>RSPWARWFPKTLPCDVTLDVSKNHVIVDCTDKHLTEIPGGIPTNTTNLTLTINHIPDISPASFHRLVHLVEIDFRCNCVPIRLGSKSNMCPRRLQIKPRSFSGLTYLKSLYLDGNQLLEIPQGLPPSLQLLSLEANNIFSIRKEQLTELANIEILYLGQNCYYRNPCYVSYSIEKDAFLNLTKLKVLSLKDNNVTTVPTVLPSTLTELYLYNNMIAEIQEDDFNNLNQLQILDLSGNCPRCYNAPFPCTPCKNNSPLQIPVNAFDALTELKVLRLHSNSLQHVPPRWFKNINNLQELDLSQNFLAKEIGDAKFLHFLPNLIQLDLSFNFELQVYRASMNLSQAFSSLKSLKILRIRGYVFKELKSFQLSPLHNLQNLEVLDLGTNFIKIANLSMFKQFKRLKVIDLSVNKISPSGDSLVPRGSSNARTSVESYEPQVLEQLYYFRYDKYARSCRFKNKEASFTSVQESCYKYGQTLDLSKNSIFFIKSSDFQHLSFLKCLNLSGNLISQTLNGSEFQPLAELRYLDFSNNRLDLLHSTAFEELRKLEVLDISSNSHYFQSEGITHMLNFTKNLKVLQKLMMNDNDISSSTSRTMESESLRTLEFRGNHLDVLWRDGDNRYLQLFKNLLKLEELDISKNSLSFLPSGVFDGMPPNLKNLSLAKNGLKSFIWEKLRYLKNLETLDLSHNQLTTVPERLSNCSRSLKNLILKNNQIRSLTKYFLQDAFQLRYLDLSSNKIQMIQKTSFPENVLNNLKMLLLHHNRFLCTCDAVWFVWWVQHTEVTIPYLATDVTCVGPGAHKGQSVISLDLYTCELDLTNEFLVPR[2x]

TLR7 recognizes pathogenic single-stranded RNAs (ssRNAs) and plays a crucial role in the innate immune response to viral infections, such as human immunodeficiency virus 1 and influenza virus. The activated TLR7 dimer contains two distinct ligand-binding sites. Small-molecule agonists, including imiquimod, guanosine and 2’,3’-cGMP bind to site 1 in the dimerization interface and directly induce the formation of the activated TLR7 dimer, while uridine-containing ssRNAs bind to site 2 and allosterically enhance the binding affinity of site 1 ligands for TLR73,4. Using cryo-electron microscopy (cryo-EM) combined with X-ray crystallography, we reveal that the structural equilibrium between open and closed conformations that underlies TLR7 antagonism.

We have previously reported a series of 8-oxoadenine derivatives (8-OAs) represented by Cpd-1, Cpd-2, and Cpd-3 as specific TLR7 agonists. We confirmed the binding mode of 8-OAs by crystallography. The potent agonist Cpd-3 induced almost complete dimerization under both neutral and acidic conditions. The TLR7/Cpd-3 complex exclusively adopted a closed-form conformation which is in good agreement with the crystal structure. Three agonists Cpd-1, Cpd-2, and Cpd-3 had higher binding energy in the closed form than the open form. Cpd-1, Cpd-2, Cpd-3 and other known TLR7 agonists induce a closed form structure which activates TLR7.>HRPLNPAMVAFSNDPLLNDLALNSSYSLLFAVNNMKSEKSAEQFYGKMDNQKMLDLVRASSTKIDFDPTLLPTMNSNPATYQGKRKNLVILLQESLGAQFVGSLGGLPLTPNLDELMQEGWQFTQMYATGTRSVRGIEAVTTGFPPSPSRAVVKLSKSQTGFFTIADLLKEQGYHTQFIYGGEANFDNMKTFFFGNGFDQIVEEKNYTNPGFVGSWGVSDEDLYNKADEEFERLSKGDKPFFSLVFTSSNHSPYEYPEGKIEQYDSEHMTRNNAVKYSDYALGTFFDKAKKSSYWDDTIFIVIADHDARVFGANLVPVKHFHIPALIIGKDIQPRKDDRIANNIDMPPTLLSLIGVDAKTPMIGRDLTKPLAREDERAMMQYDKNFGYLTRDNLVVLSPGEKVSTMEYDFESQTMKPLEVDESVIDRAKANALFASK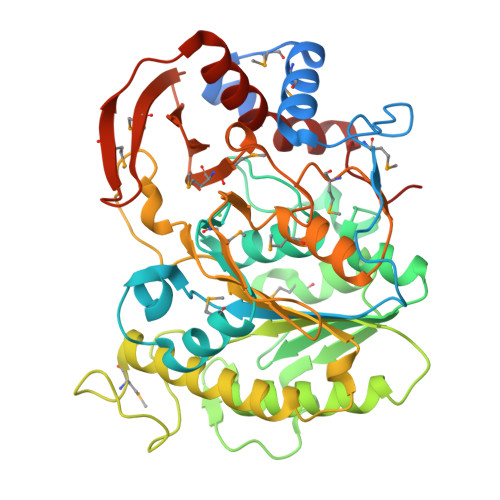AYQNNWYSSKRTN[2x]>HMGSSPLRRVLAELNRIPSSRRRAARLFEWLIAPMPPDHFYRRLWEREAVLVRRQDHTYYQGLFSTADLDSMLRNEEVQFGQHLDAARYINGRRETLNPPGRALPAAAWSLYQAGCSLRLLCPQAFSTTVWQFLAVLQEQFGSMAGSNVYLTPPNSQGFAPHYDDIEAFVLQLEGRKLWRVYRPRAPTEELALTSSPNFSQDDLGEPVLQTVLEPGDLLYFPRGFIHQAECQDGVHSLHLTLSTYQRNTWGDFLEAILPLAVQAAMEENVEFRRGLPRDF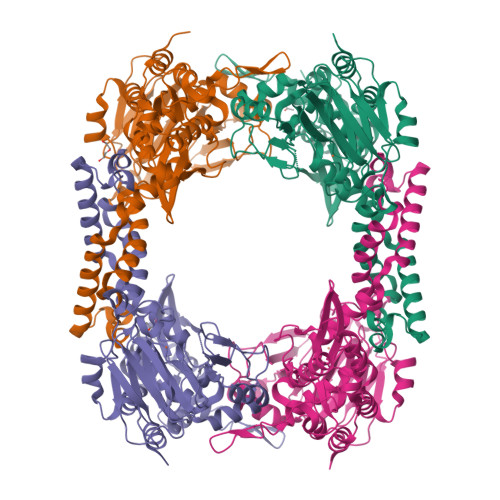MDYMGAQHSDSKDPRRTAFMEKVRVLVARLGHFAPVDAVADQRAKDFIHDSLPPVLTDRERALSVYGLPIRWEAGEPVNVGAQLTTETEVHMLQDGIARLVGEGGHLFLYYTVENSRVYHLEEPKCLEIYPQQADAMELLLGSYPEFVRVGDLPCDSVEDQLSLATTLYDKGLLLTKMPLALN[4x]>[2x]MVEVVSVSRHDRWRGVYVVELEDGSLRIATKNLVPGQRVYGERIFRYNGEEYREWNAYRSKLAAALLKGLIELPVKEGDRILYLGIASGTTAS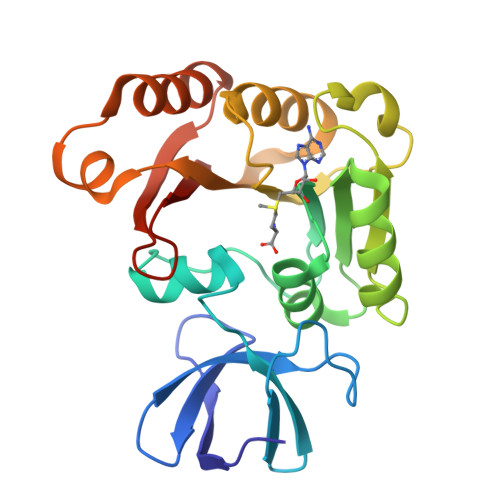HMSDIIGPRGRIYGVEFAPRVMRDLLTVVRDRRNIFPILGDARFPEKYRHLVEGVDGLYADVAQPEQAAIVVRNARFFLRDGGYMLMAIKARSIDVTTEPSEVYKREIKTLMDGGLEIKDVVHLDPFDRDHAMIYAVMRR Elp3 acts as the catalytic subunit, but the loss of any of the six subunits results in hypo-modified U34 tRNAs in yeast, indicating that the complete integrity of the complex is important for its function. The enzymatically active Elp3 subunit of Elongator contains two functional domains, utilizes multiple cofactors, and conducts a unique uridine base modification specifically found only at the wobble base position of tRNAs. The two domains form a cleft that contains several highly conserved basic residues, which bind and accommodate the tRNA anticodon stem loop (ASL). The current model of a radical based Elp3-mediated cm5-modification reaction is proposed as follows (i) Elp3 recruits SAM and cleaves it to generate a 5’deoxyadenosine radical (5’-dA) in the rSAM domain, (ii) Elp3 hydrolyzes acetyl-CoA in the KAT domain and (iii) an acetyl radical is formed by the products of the two domains and (iv) is transferred onto the C5 position of U34 in the bound tRNA molecule.

We used full length and truncated versions of purified MinElp3 in crystallization trials and obtained well-diffracting crystals for monomeric MinElp3Δ1–19, MinElp3Δ1–46, and MinElp3Δ1–54. We solved their structures using a poly-alanine model of DmcElp3 via molecular replacement at 1.9 Å, 1.9 Å, and 2.1 Å resolution, respectively. Although all three versions contained various lengths of the N-terminus and also showed no signs of degradation, we could observe interpretable electron density only starting from residue V72 in all collected and refined datasets. The overall structure and domain arrangement and interface between the rSAM and KAT domains of MinElp3 are almost identical to DmcElp3. The main difference relates to the Fe–S cluster loop region (aa 87–123) and the Fe–S cluster itself, which were both completely unstructured in all monomeric MinElp3s. We previously identified a Zn-binding motif in the central linker region between the two domains that is coordinated by three cysteine residues, which are strictly conserved in bacterial and archaeal but missing in eukaryotic Elp3s. In our MinElp3 structures, we could not locate any bound Zn-ions and instead observed the formation of a disulfide bond between C384 and C389. Nevertheless, the equivalent sequence still obtains an almost identical conformation, indicating that zinc might simply contribute structural integrity in anaerobic bacteria. In addition, we observed that the acetyl-CoA blocking loop (aa 466–486) is positioned outside of the acetyl-CoA binding pocket, interacting with the last visible residues of the N-terminus and also contacting a neighboring symmetry mate. Using our DmcElp3-DCA structure as a reference model, we are able to show that acetyl-CoA would also fit seamlessly into the active site of MinElp3, indicating an almost identical ligand coordination and active site organization.

> GAMATEEEKKILIPILRKKPVRTISGVAVVAVMTSPAKCPHGKCIFCPGGLDSVFGDVPQSYTGREPATMRGLMFNFDPYLQTRARIEQLEKVGHPTDKIELIIMGGTFPAREIEYQDWFIKRCLDAMNERESKSLEEAQKINETAKHRCVALCIETRPDYCSEKEINQMLKLGATRVELGVQSIYNEILKLCKRGHSVEDTIKATQLLKDSGLKVSYHLMPGMPGSSIEMDKKMFKEIFTNPDFMPDMVKIYPCLVIEGTELYEMWKRGEFKPYREEEAIEVISYAKSIMPKWVRTSRIQRDIPATVIVDGVKKSNLGELVYKYMEKKGLRCRCIRCREVGHVYYKKGILPDPEHIKLVREDYEASGGTEIFLSFEDVKNDILIAFLRLRDPYKPFRKEIDDKTMLVRQLHVFGWEKALTRDIKEVSWQHMGYGRMLMKEAERIAKEEFGKKKILVTSGIGVREYYRKLGYKRVGAYMGKEL The Tn1549 conjugative transposon propagates resistance to the antibiotic vancomycin used for severe drug-resistant infections. The DNA cleavage and joining reactions required for CTn transposition are carried out by a transposase enzyme called integrase (Int). Most known CTns, including the Tn916-like family, have Y-transposases that use a conserved tyrosine residue to attack a phosphorous atom in the DNA backbone. Int contains 3 functional domains: an arm-binding domain (AB), a core DNA binding domain (CB), and a catalytic domain (CAT).

Concerning the nucleophile tyrosine, Int contains two tyrosine residues located near the active site: Y379 at the end of αL points toward the scissile phosphate, and Y380 in the subsequent loop that threads away from the active site sits in a snug pocket on the interface of the two protein subunits. Hydrophobic interactions and hydrogen bonds keep Y380 in a buried position, where it is unable to act as a nucleophile in DNA cleavage. To explore the two tyrosines’ roles in DNA cleavage and recombination, we generated single and double point mutants of Int82N, substituting one or both with phenylalanine that cannot cleave DNA. Both single mutants cleaved DNA in vitro, whereas the double mutant was completely inactive. However, in strand exchange Y380F was completely inactive, whereas Y379F was active as the unmutated protein. Thus, while both Y379 and Y380 can perform DNA cleavage, only cleavage via Y380 can proceed to strand exchange. In agreement, in vivo assays in E.coli showed that Y380 is critical for Tn1549 excision, whereas Y379 is dismissible (Lambertsen et al., 2018).

>[2x]SMTVCQLYAKQIRHRGNVKHNTKLGRERLMRILEQDRLGSCPIDSVKLSDAKEWALRMKEKGLSYKTINNDKRSLKAAFYTAIQDDCIRKNPFDFQLSDVLDDDTEPKVPLTPAQEESFLSFIQGDKVYQKHYDAIVILLGTGLRISELCGLTDKDLDFENRVIIVSHQLLRNTGVGYYIDEPKTQSGVRKIPMNEEVYQAFQRVIKNRKGAKPFIIDGYANFLFLKQNGYPMTAVDYGGMFGRLVKKYNKSHEEALPKTTTPHAMRHTFCTRLANAGMNPKALQYIMGHSNITMTLNFYAHATFDSARAEMERLAA> GHMVPELKQISREEAMRLGPGWSHSCHAMLYAANPGQLFGRIPMRFSVLMQMRFDGLLGFPGGFVDRRFWSLEDGLNRVLGLGLGGLRLTEADYLSSHLTEGPHRVVAHLYARQLTLEQLHAVEISAVHSRDHGLEVLGLVRVPLYTQKDRVGGFPNFLSNAFVSTAKYQLLF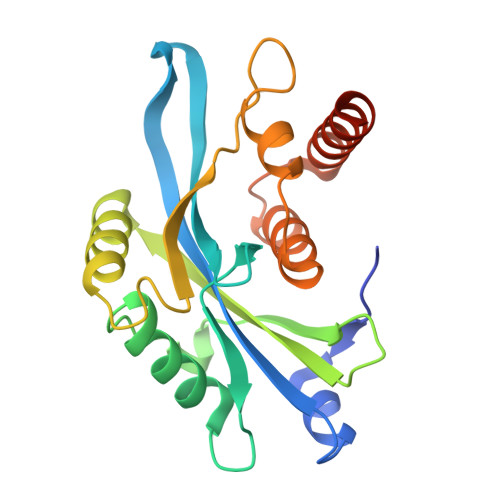ALKVLNMMPSEKLAEALASATEKQKKALEKLLPPSS> GSYGPVFVQEPDDVIFPTDSDEKKVALNCEVRGNPSPSYRWLRNGTEIALESDYRYS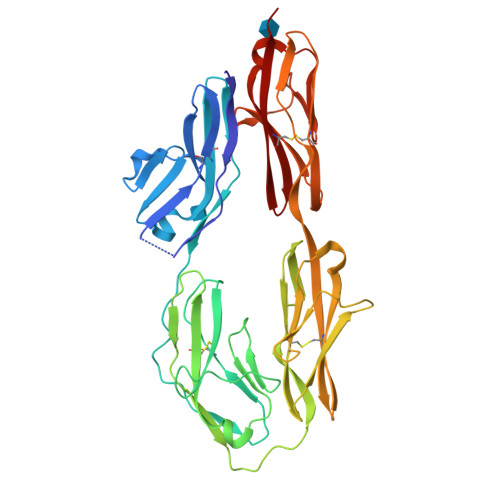LIDGTFIISNPSELRDSGLYQCLATNSFGSILSREATLQFAYLGNFSGRTRSAVSVREGQGVVLMCSPPPHSPEIIYSWVFNEFPSFVAEDSRRFISQETGNLYISKVQTSDVGSYICLVKNAVTNARVLSPPTPLTLRNDGVMGEYEPKIEVHFPFTVTAAKGTTVKMECFALGNPVPTITWMKVNGYIPSKSRLRKSQAVLEIPNLQLDDAGIYECTAENSRGKNSFRGQLQIFTYPHWVQKLNDTQLDSGSPLQWECKATGKPRPTYRWLKNGAPLLPQSRVDTVNGILAIQSVNQSDAGMYQCLAENKYGAIYASAELKILAS2-(6-chloranyl-7-cyclopropyl-thieno[3,2-d]pyrimidin-4-yl)sulfanylethanoic 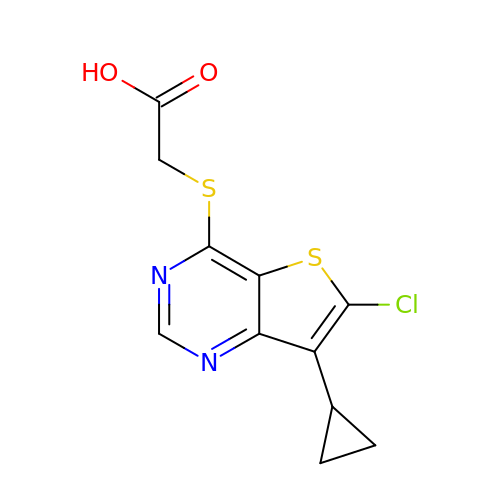acid | C11 H9 Cl N2 O2 S2 | LJYRIWUQISYYHA-UHFFFAOYSA-N>[3x]MIQGVIQKIAGPAVIAKGMLGARMYDICKVGEEGLVGEIIRLDGDTAFVQVYEDTSGLKVGEPVVSTGLPLAVELGPGMLNGIYDGIQRPLERIREKTGIYITRGVVVHALDREKKWAWTPMVKPGDEVRGGMVLGTVPEFGFTHKILVPPDVRGRVKEVKPAGEYTVEEPVVVLEDGTELKMYHTWPVRRARPVQRKLDPNTPFLTGMRILDVLFPVAMGGTAAIPGPFGSGKTVTQQSLAKWSNADVVVYVGCGERGNEMTDVLVEFPELTDPKTGGPLMHRTVLIANTSNMPVAAREASIYVGVTIAEYFRDQGFSVALMADSTSRWAEALREISSRLEEMPAEEGYPPYLAARLAAFYERAGKVITLGGEEGAVTIVGAVSPPGGDMSEPVTQSTLRIVGAFWRLDASLAFRRHFPAINWNGSYSLFTSALDPWYRENVAEDYPELRDAISELLQREAGLQEIVQLVGPDALQDAERLVIEVGRIIREDFLQQNAYHEVDAYCSMKKAYGIMKMILAFYKEAEAAIKRGVSIDEILQLPVLERIGRARYVSEEEFPAYFEEAMKEIQGAFKALA;>MDLLKKEYTGITYISGPLLFVENAKDLAYGAIVDIKDGTGRVRGGQVIEVSEEYAVIQVFEETTGLDLATTSVSLVEDVARLGVSKEMLGRRFNGIGKPIDGLPPITPEKRLPITGLPLNPVARRKPEQFIQTGISTIDVMNTLVRGQKLPIFSGSGLPANEIAAQIARQATVRPDLSGEGEKEEPFAVVFAAMGITQRELSYFIQEFERTGALSRSVLFLNKADDPTIERILTPRMALTVAEYLAFEHDYHVLVILTDMTNYCEALREIGAAREEIPGRRGYPGYMYTDLATIYERAGVVEGKKGSVTQIPILSMPDDDRTHPIPDLTGYITEGQIQLSRELHRKGIYPPIDPLPSLSRLMNNGVGKGKTREDHKQVSDQLYSAYANGVDIRKLVAIIGEDALTENDRRYLQFADAFERFFINQGQQNRSIEESLQIAWALLSMLPQGELKRISKDHIGKYYGQKLEEIWGAPQALD[3x];> MSQVSPTRMNLLQRRGQLRLAQKGVDLLKKKRDALVAEFFGLVREAMEARKALDQAAKEAYAALLLAQAFDGPEVVAGAALGVPPLEGVEAEVENVWGSKVPRLKATFPDGALLSPVGTPAYTLEASRAFRRYAEALIRVANTETRLKKIGEEIKKTTRRVNALEQVVIPGIRAQIRFIQQVLEQREREDTFRLKRIKGKIEAREAEEEGGRPNPQVEIGAGL;> MAVIADPETAQGFRLAGLEGYGASSAEEAQSLLETLVERGGYALVAVDEALLPDPERAVERLMRGRDLPVLLPIAGLKEAFQGHDVEGYMRELVRKTIGFDIKL;>MTGGLVLNAISRAGGAMGGLGLIKSLAEKEKQLLERLEAAKKEAEERVKRAEAEAKALLEEAEAKAKALEAQYRERERAETEALLARYRERAEAEAKAVREKAMARLDEAVALVLKEVLP[2x];>MSKLEAILSQEVEAEIQALLQEAEAKAEAVKREAEEKAKALLQARERALEAQYRAALRRAESAGELLVATARTQARGEVLEEVRRRVREALEALPQKPEWPEVVRKLALEALEALPGAKALVANPEDLPHLEAMARERGVELQAEPALRLGVRAVGAEGKTQVENSLLARMDRAWDAMSSKVAQALWG[2x];> MADDFAYLNARVRVRRGTLLKESFFQEALDLSFADFLRLLSETVYGGELAGQGLPDVDRAVLRTQAKLVGDLPRLVTGEAREAVRLLLLRNDLHNLQALLRAKATGRPFEEVLLLPGTLREEVWRQAYEAQDPAGMAQVLAVPGHPLARALRAVLRETQDLARVEALLAKRFFEDVAKAAKGLDQPALRDYLALEVDAENLRTAFKLQGSGLAPDAFFLKGGRFVDRVRFARLMEGDYAVLDELSGTPFSGLSGVRDLKALERGLRCVLLKEAKKGVQDPLGVGLVLAYVKEREWEAVRLRLLARRAYFGLPRAQVEEEVVCP

The V/A ATPase from the thermophilic eubacterium Thermus thermophilus (Tth) is one of the best characterized rotary ATPases. The a-subunit is connected to the A3B3 stator in the V1 domain by two peripheral EG stalks which form a peripheral stator apparatus (A3B3E2G2a1). In addition, the dodecamer c ring composed of two transmembrane α-helices, the d-subunit and the DF shaft constitute the central rotor complex (D1F1d1c12), which rotates relative to the surrounding stator apparatus. The proton motive force generated by respiratory complexes drives proton translocation through a proton pathway made up of both the a-subunit and the c12 ring.

To overcome structural heterogeneity, we employed masked refinement with V1EGd soft mask for the hydrophilic region. The map of state1 at 4.7 Å resolution produced a well defined atomic model by MDFF, particularly in the V1 region. The three AB pairs in A3B3 adopt three different conformations known as ‘open’, ‘closed’, and ‘semi-closed’, as seen in previously reported structures of the F1 and V1 complexes. In this model, strong positive density was observed near the P-loop in two AB pairs; the ‘closed’, and ‘semi-closed’ state. A molecule of ADP fits well into each density. There is no obvious density adjacent to the β-phosphate of the fitted ADP at each region, suggesting these densities represent bound ADP and not ATP. No density is observed near the P-loop in the AB pair in the ‘open’ state. The model at a resolution of 4.7 Å for the hydrophilic region provides detailed structural information for the three nucleotide binding sites composed of the AB pairs, in the open, closed and semi-closed conformations. Thus, we conclude that the EM map presented here corresponds to the ADP inhibited state after phosphate has detached from the semi-closed site leaving ADP still bound. Our higher resolution model of state1 reveals that there are close interactions between E/160–164 of E-subunits and B/5–9 of B-subunit, where rigid β-sheet structures are formed.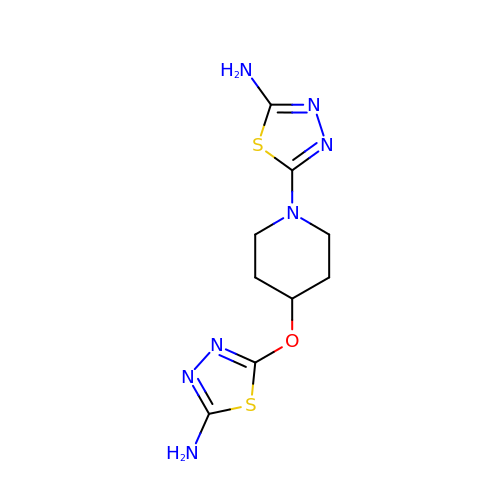5-{4-[(5-amino-1,3,4-thiadiazol-2-yl)oxy]piperidin-1-yl}-1,3,4-thiadiazol-2-amine | C9 H13 N7 O S2 | RUDRLRZJXZZCQT-UHFFFAOYSA-N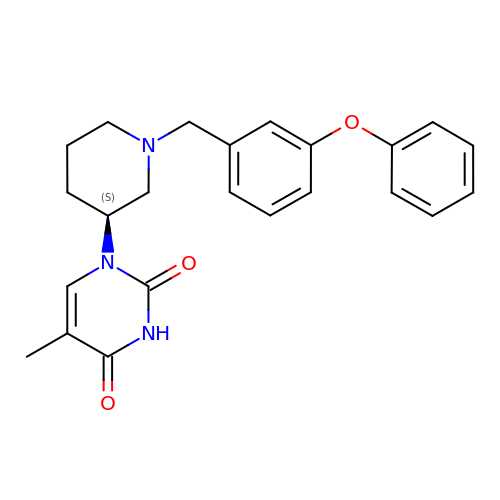5-methyl-1-[(3~{S})-1-[(3-phenoxyphenyl)methyl]piperidin-3-yl]pyrimidine-2,4-dione | C23 H25 N3 O3 | UVSXXFBEAJISCP-IBGZPJMESA-N> MGPQRRLSPAGAALLWGFLLQLTAAQEAILHASGNGTTKDYCMLYNPYWTALPSTLENATSISLMNLTSTPLCNLSDIPPVGIKSKAVVVPWGSCHFLEKARIAQKGGAEAMLVVNNSVLFPPSGNRSEFPDVKILIAFISYKDFRDMNQTLGDNITVKMYSPSWPNFDYTMVVIFVIAVFTVALGGYWSGLVELENLKAVTTEDREMRKKKEEYLTFSPLTVVIFVVICCVMMVLLYFFYKWLVYVMIAIFCIASAMSLYNCLAALIHKIPYGQCTIACRGKNMEVRLIFLSGLCIAVAVVWAVFRNEDRWAWILQDILGIAFCLNLIKTLKLPNFKSC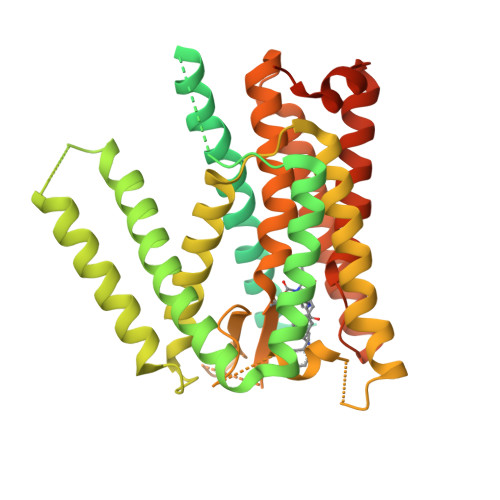VILLGLLLLYDVFFVFITPFITKNGESIMVELAAGPFGNNEKLPVVIRVPKLIYFSVMSVCLMPVSILGFGDIIVPGLLIAYCRRFDVQTGSSYIYYVSSTVAYAIGMILTFVVLVLMKKGQPALLYLVPCTLITASVVAWRRKEMKKFWKGNSYQMMDHLDCATNEENPVISGEQIVQQ> MKKWFPALLFSLCVSGESSAWNNIVFYSLGDVNSYQGGNVVITQRPQFITSWRPGIATVTWNQCNGPGFADGFWAYYREYIAWVVFPKKVMTQNGYPLFIEVHNKGSWSEENTGDNDSYFFLKGYKWDERAFDAGNLCQKPGETTRLTEKFDDIIFKV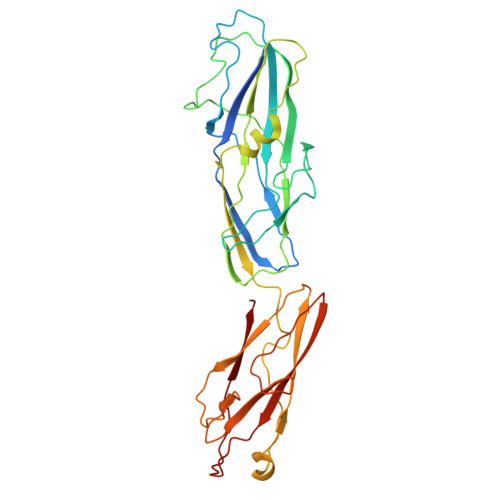ALPADLPLGDYSVKIPYTSGMQRHFASYLGARFKIPYNVAKTLPRENEMLFLFKNIGGCRPSAQSLEIKHGDLSINSANNHYAAQTLSVSCDVPANIRFMLLRNTTPTYSHGKKFSVGLGHGWDSIVSVNGVDTGETTMRWYKAGTQNLTIGSRLYGESSKIQPGVLSGSATLLMILP> MSKENQNVVLVSVEGERFVVDRKIAERSLLLKNYLQDLNSGDLHDDNDADDDEDDEEDGDDEIVMPVPNVRSSVLQKVIEWAVHHKDSNFPDEDDDDSRKAAPVDPWDREFLKVDQEMLYEIILAANYLNIKPLLDAGCK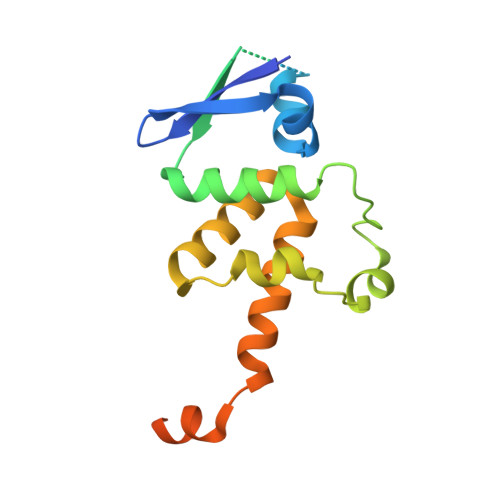VVAEMIRGRTPEEIRRTFNIVNDFTPEEEAAIRRENEWAEDR> MGSSHHHHHHSSGRENLYFQGMTKLKAPAVLAYSRKINPTNALMFAVNWSDRDNTTAVMVGTKTVAGTQSVRG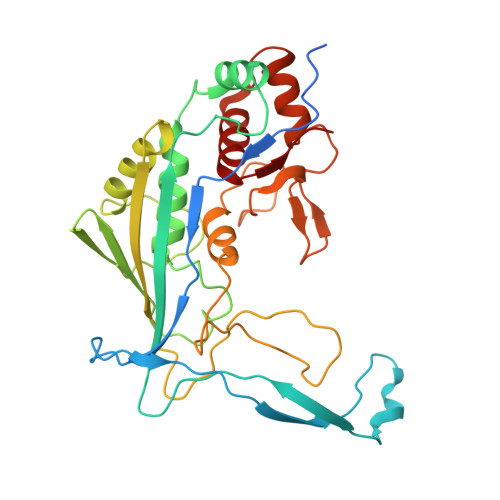NPNDADKGNIQTVNFANLPHNKNTLLVKYNVKFVGDVFKAELGGGEYSNTLQTALENTDFGTLAYRYVYNIAAGRTLWRNRVGAESIETVITVNDQTFTFSDLLVNEFDEDVDVAEIADMVAGVLSGEGFVTLKVEHYMLLGEGSEVFPSQEFVENSKLSKQLFDLNGQAAMHDQKIGNAIRTIDTWYEDATTPIAVEPYGSVVRNGVAYRAGNKTDLFTLMDGAVNGKSLTEEDQMFVTANLIRGGVFGGGKD>[3x]GMPNFSKNEEVLFSAVNEIFEEKIPFNKIIGLKVRFISPEQVKLSFEMRDELIGNAIRRMLYGGVISSAIDMTAGLAAF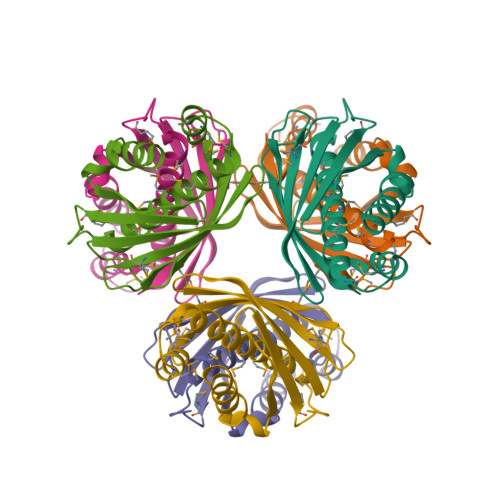MGFQEKMSGKPMEEKLAMIGRLSTMSLHVEYLRPGLGREFVCTGYNVRTGNKVAVIRTELMNDQDELIAVGSVSYILV N-{3-[5-chloro-2-(difluoromethoxy)phenyl]-1-methyl-1H-pyrazol-4-yl}pyrazolo[1,5-a]pyrimidine-3-carboxamide 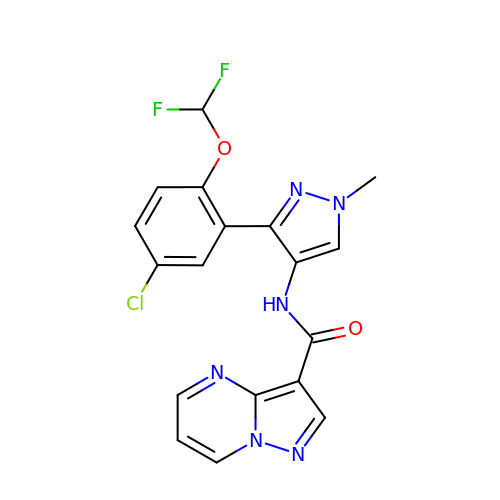| C18 H13 Cl F2 N6 O2 | CJXPNZXEEPSZHK-UHFFFAOYSA-N6-AMINOURIDINE 5'-MONOPHOSPHATE | C9 H14 N3 O9 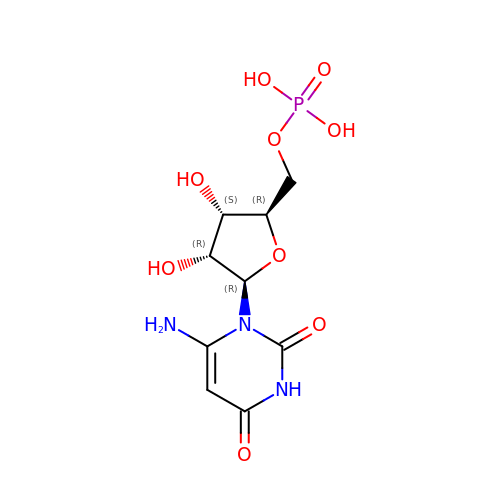P | DUFXRFNPGXQQOI-YXZULKJRSA-N> MSDTPYKADLSRVHWAGSNSDVDIHLEIFEGDVDSGFMYNSFFRGNSSYVSVQDQSNQARIDRMNTVTIKGRTPGQKLDRESVKNDKLVITVDTVTYASTVMDWQDDWTSPDRWAEIGAQHGYQHARLFD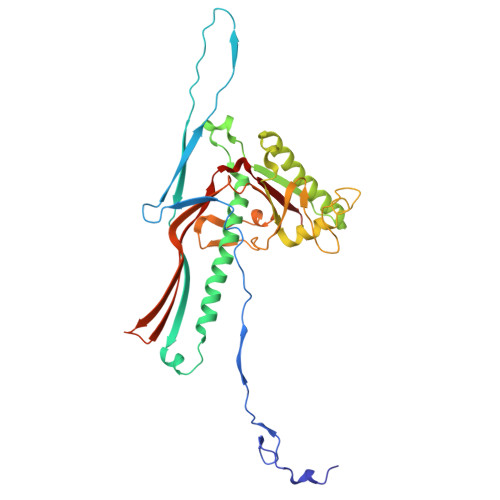TAHLIQIIKARKWIAPADLKPAFFDGKEYTAAYNADRELFAANIIDAHRQGIEEMVRRDLGGSLTEFITVVSPYVFGLLLDSKKLVNVDYSAGNGNFAERRVGMVNGVRIVESARFPAAAGTSPLGAAFTVDADDVACQMVVYHPKMTLVTVEAKPLATNKYPDNPNFSDILDSFTLYTVGQRRPDTSFAVKLTNLP>MAEAQNDPLLPGYSFNAHLVAGLTPIEANGVLDFFIDRPLGMKG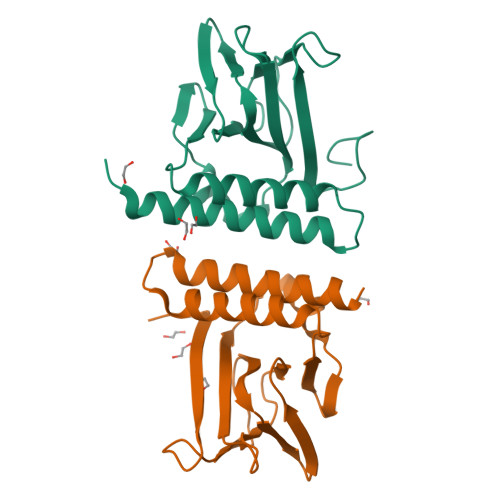YILNLTIRGQGVVKNQGREFVCRPGDILLFPPGEIHHYGRHPEAREWYHQWVYFRPRAYWHEWLNWPSIFANTGFFRPDEAHQPHFSDLFGQIINAGQGEGRYSELLAINLLEQLLLRRMEAINESLHPPMDNR[5x]> MRKQIHPLILFSFFGIMMFILIINRPLNDSQSFKTKSNIAQIEAQALKHLDKPIIDLSGWQRPEEINYDALSQNISGAIVRVHSGAQTTKENDASFINGIDKAYKSHITELQKRNVPVAVYAYVAGKSVQEMEKAAEVFYNAASPYSPSYYWLDVEDKTMSNMNEGVENFRAKLASLGAKNIGIYVGVYFMEEHSIDTGKFTSVWIPSYGSDSGFLESSPKTDL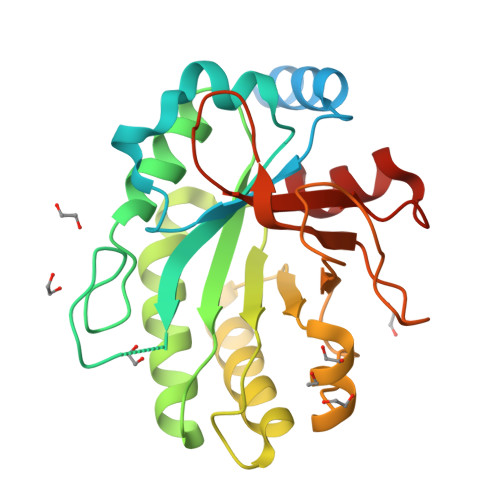DYDIHQYTSKGKIAGFDHDLDINVISPLKNKEETFRKLFLKP> MDETGKELVLVLYDYQEKSPRELTVKKGDIL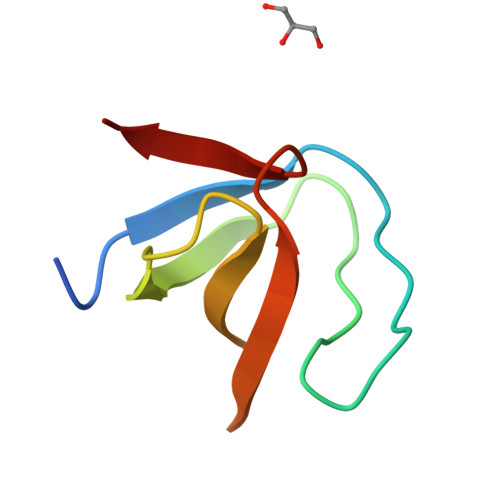TLLNSTNKDWWKIEVNDRQGFVPAAYLKKLD Amplification of piRNA in the ping-pong cycle requires assembly of a tertiary complex scaffolded by Krimper, which simultaneously binds the N-terminal regions of Aub and Ago3. To promote generation of new piRNA, Krimper uses its two Tudor domains to bind Aub and Ago3 in opposite modification and piRNA-loading states. In addition to its self-interacting N-terminal region, Krimper contains two extended Tudor domains: eTud1(272-512) and eTud2 (562-746). Overall, our results reveal that the two Tudor domains of Krimper have distinct architectures that are responsible for the differential binding of two PIWI proteins.

In the 2.1 Å eTud1 apo structure, crystals belong to the P212121 space group with two monomers in the asymmetric unit. The overall structure is similar to eTud2 apart from the C-terminal region (484-511aa) that forms a long α-helical fold that inserts into the narrow interface between the Tudor and SN-like subdomains. We named this novel C-terminal helical topology the “latch helix”. The latch helix is stabilized through formation of extensive hydrogen bondings and salt bridge interactions with its amphipathic concave binding site within eTud1. Furthermore, eTud1 possesses a ‘latch helix’ that must move out of the cleft to allow Ago3 binding providing a potential regulatory mechanism. First, the N-terminus of eTud1 contains a long-loop (spanning amino acids 272-300) connecting and interacting with both the Tudor and the SN-like subdomains. Pro292 within this N-terminal loop forms a CH-π interaction with Tyr365, Glu297 in the loop region forms a hydrogen bonding with the backbone of Ser387, Arg300 in the loop forms a hydrogen bond and salt bridge interactions with Asp394, while Tyr304 in the loop forms cation-π interaction with Arg428 in the SN-like domain. All these intramolecular interactions help to stabilize the overall structure of eTud1. Although the overall topology of eTud1 is similar to other extended Tudor domains, eTud1 has its own unique folding and recognition characteristics. The unusual binding preference of eTud1 is reflected in its non-canonical binding pocket, which lacks three of the four conserved aromatic residues.

>[2x]SASIEKVNKLPKSPRNRFLLPPKGGTETTRRDIYNQILKDMAAFPENTIVTAVLASVDVTDNCAYVAKWDESSDRIKKVLQRQLPLQELDQLPDYGDIFAVLDSINNIITRITINSSSAGGGYDAYLIDFGEHIHFDGNETIFKLPDDIKRLPAQAIRCDLINCDIANMHCFVNTYIKIRVHENNNSTLVAEPVIDRLSRPTKTNTTKYPAGITEDDMAMLNEIDESTSDPLKAVLGFRPKD> MKV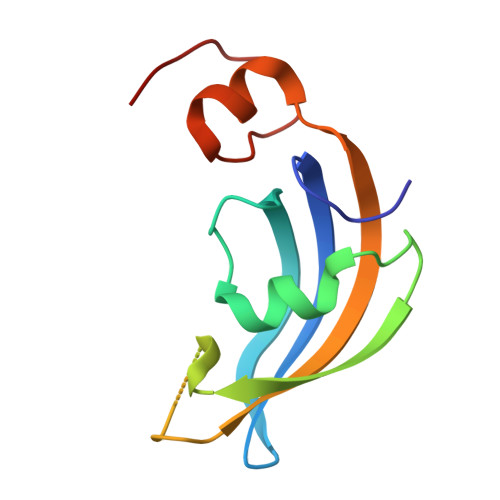GQDKVVTIRYTLQVEGEVLDQGELSYLHGHRNLIPGLEEALEGREEGEAFQAHVPAEKAYGATGHPGIIPPHATLDFQVEVVKVREATPEELLHGHAHPSGHHHHHH>MVGLIWAQATSGVIGRGGDIPWRLPEDQAHFREITMGHTIVMGRRTWDSLPAKVRPLPGRRNVVLSRQADFMASGAEVVGSLEEALTSPETWVIGGGQVYALALPYATRCEVTEVDIGLPREAGDALAPVLDETWRGET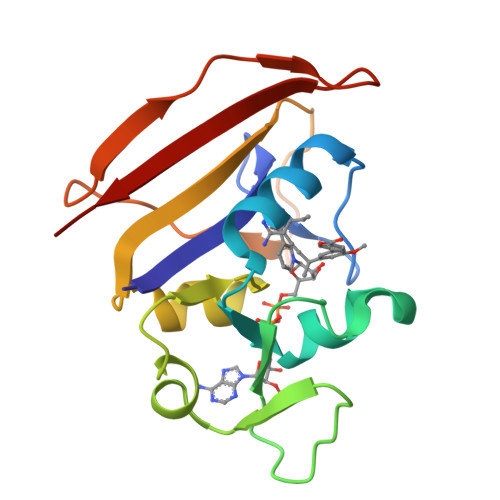GEWRFSRSGLRYRLYSYHRS[4x]> SKYGLQDSDEEEEEHPSKTSTKKLKTAPLPPASQTTPLQMALNGKPAPPPQSQSPEVEQLGRVVELDSDMVDITQEPVLDTMLEESMPEDQEPVSASTHIASSLGINPHVLQIMKASLLTDEEDVDMALDQRFSRLPSKADTSQEICSPRLPISASHSSKTRSLVGGLLQSKFTSGAFLSPSVSVQECRTPRAASLMNIPSTSSWSVPPPLTSVFTMPSPAPEVPLKTVGTRRQLGLVPREKSVTYGKGKLLMDMALFMGRSFRVGWGPNWTLANSGEQLNGSHELENHQIADSMEFGFLPNPVAVKPLTESPFKVHLEKLSLRQRKPDEDMKLYQTPLELKLKHSTVHVDELCPLIVPNLGVAVIHDYADWVKEASGDLPEAQIVKHWSLTWTLCEALWGHLKELDSQLNEPREYIQILERRRAFSRWLSCTATPQIEEEVSLTQKNSPVEAVFSYLTGKRISEACSLAQQSGDHRLALLLSQFVGSQSVRELLTMQLVDWHQLQADSFIQDERLRIFALLAGKPVWQLSEKKQINVCSQLDWKRSLAIH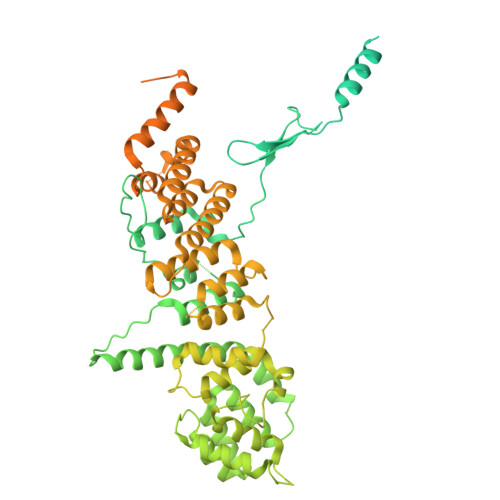LWYLLPPTASISRALSMYEEAFQNTSDSDRYACSPLPSYLEGSGCVIAEEQNSQTPLRDVCFHLLKLYSDRHYDLNQLLEPRSITADPLDYRLSWHLWEVLRALNYTHLSAQCEGVLQASYAGQLESEGLWEWAIFVLLHIDNSGIREKAVRELLTRHCQLLETPESWAKETFLTQKLRVPAKWIHEAKAVRAHMESDKHLEALCLFKAEHWNRCHKLIIRHLASDAIINENYDYLKGFLEDLAPPERSSLIQDWETSGLVYLDYIRVIEMLRHIQQVDCSGNDLEQLHIKVTSLCSRIEQIQCYSAKDRLAQSDMAKRVANLLRVVLSLHHPPDRTSDSTPDPQRVPLRLLAPHIGRLPMPEDYAMDELRSLTQSYLRELAVGSL> MSRSKRDNNFYSVEIGDSTFTVLKRYQNLKPIGSGAQGIVCAAYDAILERNVAIKKLSRPFQNQTHAKRAYRELVLMKCVNHKNIIGLLNVFTPQKSLEEFQDVYIVMELMDANLSQVIQMELDHERMSYLLYQMLCGIKHLHSAGIIHRDLKPSNIVVKSDC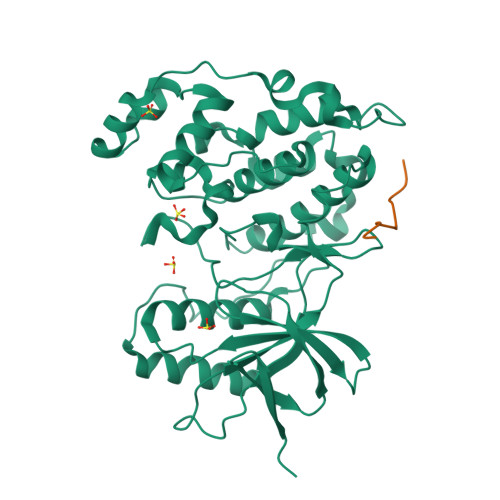TLKILDFGLARTAGTSFMMTPYVVTRYYRAPEVILGMGYKENVDIWSVGCIMGEMIKGGVLFPGTDHIDQWNKVIEQLGTPSPEFMKKLQPTVRTYVENRPKYAGYSFEKLFPDVLFPADSEHNKLKASQARDLLSKMLVIDASKRISVDEALQHPYINVWYDPSEAEAPPPKIPDKQLDEREHTIEEWKELIYKEVMDLEHHHHHH;> RPKRPTTLNLF The replication of positive-strand RNA viruses relies on virally encoded RNA-dependent RNA polymerases (RdRPs) that are capable of rapid and processive synthesis of the 7–14 kilobase viral genomes. To examine this in further detail and to validate the polymerase–RNA interactions seen in the initial poliovirus EC structures, we here present nine new coxsackievirus, rhinovirus, and poliovirus elongation complex structures at resolutions ranging from 2.1 to 2.9 Å. All the complexes feature an upstream RNA duplex that is pinched between the pinky finger and thumb domains such that the RNA exit channel is opened by ≈4 Å as compared to the polymerase alone structures. All of the complexes show the open conformation for the active site wherein the β-strands of motifs A and C are not hydrogen bonded together to fully form the RMM-fold that is commonly utilized by polymerase active sites.

Expanding on the r2 construct, the length of the upstream RNA duplex between the two ECs was shortened from 26 to 24 (r3) and 22 (r4) base pairs, and both these RNAs resulted in poliovirus EC crystals that diffracted to 2.4 Å (PV_r3) and 2.8 Å (PV_r4) resolution. Despite this common lattice organization, the different dumbbell pairs and their RNA-RNA junctions displayed a multitude of geometries in the different crystal forms; for example, the junctions in the PV EC structures range from near perfect coaxial stacking to highly disordered structures that could not be fully modeled into the electron density maps. A comparison of all the RNA-RNA junctions, shown in Figure 3, reveals geometries ranging from fairly straight and essentially canonical coaxial stacking (PV_r3, CV_r2) to slightly offset helical ends (PV_r1) to highly distorted geometries with frayed ends (PV_r5+2).

>GEIQWMRPSKEVGYPIINAPSKTKLEPSAFHYVFEGVKEPAVLTKNDPRLKTDFEEAIFSKYVGNKITEVDEYMKEAVDHYAGQLMSLDINTEQMCLEDAMYGTDGLEALDLSTSAGYPYVAMGKKKRDILNKQTRDTKEMQKLLDTYGINLPLVTYVKDELRSKTKVEQGKSRLIEASSLNDSVAMRMAFGNLYAAFHKNPGVITGSAVGCDPDLFWSKIPVLMEEKLFAFDYTGYDASLSPAWFEALKMVLEKIGFGDRVDYIDYLNHSHHLYKNKTYCVKGGMPSGCSGTSIFNSMINNLIIRTLLLKTYKGIDLDHLKMIAYGDDVIASYPHEVDASLLAQSGKDYGLTMTPADKSATFETVTWENVTFLKRFFRADEKYPFLIHPVMPMKEIHESIRWTKDPRNTQDHVRSLCLLAWHNGEEEYNKFLAKIRSVPIGRALDLPEYSTLYRRWLDSFGSSSHHHHHH[2x]>MLCEIECRALSTAHTRLIHDFEPRDALTYLEGKNIFTEDHSELISKMSTRLERIANFL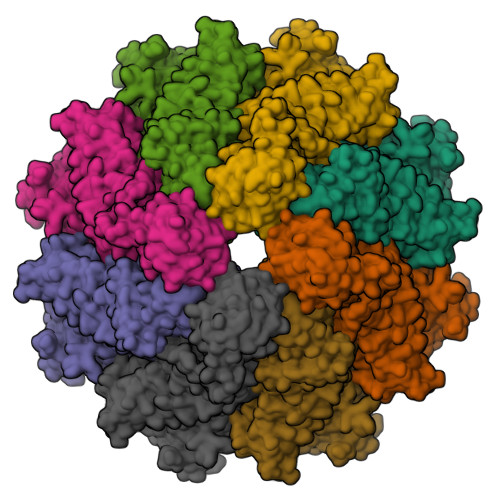RIYRRQASELGPLIDFFNYNNQSHLADFLEDYIDFAINEPDLLRPVVIAPQFSRQMLDRKLLLGNVPKQMTCYIREYHVDRVIKKLDEMCDLDSFFLFLHGRAGSGKSVIASQALSKSDQLIGINYDSIVWLKDSGTAPKSTFDLFTDILLMLKSEDDLLNFPSVEHVTSVVLKRMICNALIDRPNTLFVFDDVVQEETIRWAQELRLRCLVTTRDVEISNAASQTCEFIEVTSLEIDECYDFLEAYGMPMPVGEKEEDVLNKTIELSSGNPATLMMFFKSCEPKTFEKMAQLNNKLESRGLVGVECITPYSYKSLAMALQRCVEVLSDEDRSALAFAVVMPPGVDIPVKLWSCVIPVDICSNEEEQLDDEVADRLKRLSKRGALLSGKRMPVLTFKIDHIIHMFLKHVVDAQTIANGISILEQRLLEIGNNNVSVPERHIPSHFQKFRRSSASEMYPKTTEETVIRPEDFPKFMQLHQKFYDSLKNFACC[2x]>[3x]MRGSHHHHHHGIAGDTLGLTRPNESDAPKISIGAKDTAVVQWQGDLLAIGATENDMARDENSKFKNPLLQQLDSELNGLLSAASSEEDFSGKSGQSVNLRFPGGRITLVGLGSSASSPTSYHSLGQAAAAAAKSSQARNIAVALASTDGLSAESKINSASAIATGVVLGSFEDNRFRSESKKSTLESLDILGLGTGPEIERKIKYAEHVCAGVILGRELVNAPANIVTPAVLAEEAKKIASTYSDVISVNILDAEQCKELKMGAYLAVAAAATENPPYFIHLCFKTPTKERKTKLALVGKGLTFDSGGYNLEVGARSRIELMKNDMGGA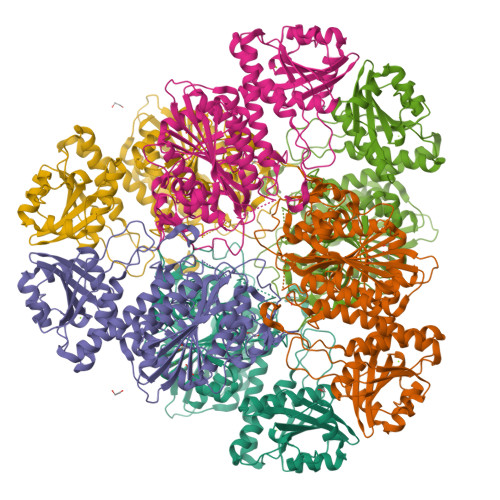AAVLGAAKALGEIRPSRVEVHFIVAACENMISAEGMRPGDIVTASNGKTIEVNNTDAEGRLTLADALIYACNQGVEKIIDLATLTGAIMVALGPSVAGAFTPNDDLAREVVEAAEASGEKLWRMPMEESYWESMKSGVADMINTGPGNGGAITGALFLKQFVDEKVQWLHLDVAGPVWSDEKKNATGYGVSTLVEWVLRN>MSFDIAKYPTLALVDSTQELRLLPKESLPKLCDELRRYLLDSVSRSSGHFASGLGTVELTVALHYVYNTPFDRLIWDVGHQAYPHKILTGRRDKIGTIRQKGGLHPFPWRGESEYDVLSVGHSSTSISAGIGVAIAAAKEDKQRRAVCVIGDGAITAGMAFEAMNHAGDIKPDLLVVLNDNEMSISENVGALNNHLAGGGGGGGPGTLFEELGFNYIGPVDGHDVLGLVSTLKNMRDLKGPQFLHIMTKKGRGYEPAEKDPITFHAVPKFDHTSGVLPKSSGGLPSYSKIFGDWLCETAAKDNKLMAITPAMREGSGMVEFSKKFPDRYFDVAIAEQHAVTFAAGLAIGDYKPVVAIYSTFLQRAYDQVIHDVAIQKLPVLFAIDRAGIVGADGQTHQGAFDLSFLRCIPDMVVMTPSDENECRQMLYTGYHYSDGPCAVRYPRGSGTGATLEPLASLPIGKGVVKRQGEKIAILNFGTLLPEAAAVADKLNATLVDMRFVKPLDTALILQLAGEHDALVTLEENAIMGGAGSGVNEVLMAHRRA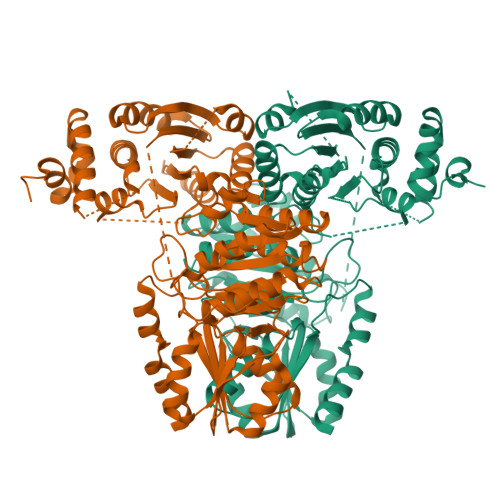VPVLNIGLPDYFIPQGTQEEIRADLGLDAAGIEAKIRDWLA[2x]> PGAVGDGPPRVDFPRSRLRFKEKLGEGQFGEVHLCEVDSPQDLVSLDFPLNVRKGHPLLV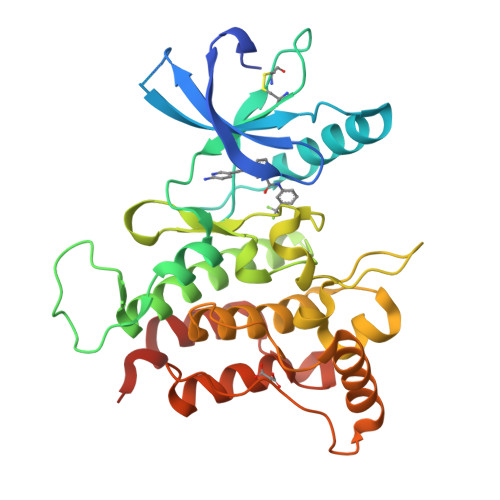AVKILRPDATKNARNDFLKEVKIMSRLKDPNIIRLLGVCVQDDPLCMITDYMENGDLNQFLSAHQLEDKAAEGAPGDPTISYPMLLHVAAQIASGMRYLATLNFVHRDLATRNCLVGENFTIKIADFGMSRNLYAGDYYRVQGRAVLPIRWMAWECILMGKFTTASDVWAFGVTLWEVLMLCRAQPFGQLTDEQVIENAGEFFRDQGRQVYLSRPPACPQGLYELMLRCWSRESEQRPPFSQLHRFLAEDALNTVHHHHHH>[2x]MTMARNWRDIRADAVAQGRVDLQRAAVAREEMRDAVLAHRLAEIRKALGHA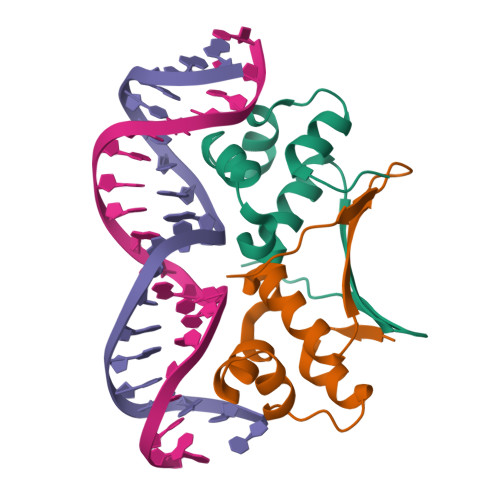RQADVAALMGVSQARVSKLESGDLSHTELGTLQAYVAALGGHLRIVAEFGENTVELTALEHHHHHH>[3x]MKLPVREFDAVVIGAGGAGMRAALQISQSGQTCALLSKVFPTRSHTVSAQGGITVALGNTHEDNWEWHMYDTVKGSDYIGDQDAIEYMCKTGPEAILELEHMGLPFSRLDDGRIYQRPFGGQSKNFGGEQAARTAAAADRTGHALLHTLYQQNLKNHTTIFSEWYALDLVKNQDGAVVGCTALCIETGEVVYFKARATVLATGGAGRIYQSTTNAHINTGDGVGMAIRAGVPVQDMEMWQFHPTGIAGAGVLVTEGCRGEGGYLLNKHGERFMERYAPNAKDLAGRDVVARSIMIEIREGRGCDGPWGPHAKLKLDHLGKEVLESRLPGILELSRTFAHVDPVKEPIPVIPTCHYMMGGIPTKVTGQALTVNEKGEDVVVPGLFAVGEIACVSVHGANRLGGN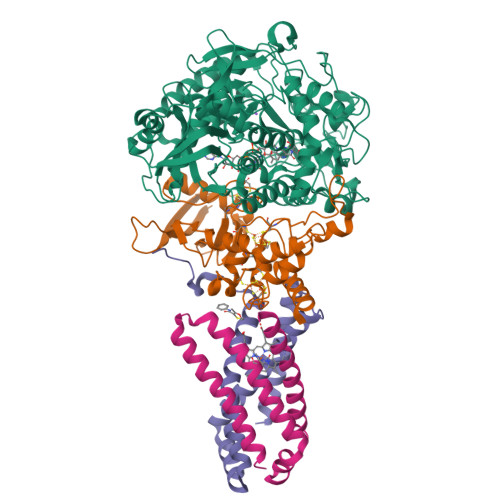SLLDLVVFGRAAGLHLQESIAEQGALRDASESDVEASLDRLNRWNNNRNGEDPVAIRKALQECMQHNFSVFREGDAMAKGLEQLKVIRERLKNARLDDTSSEFNTQRVECLELDNLMETAYATAVSANFRTESRGAHSRFDFPDRDDENWLCHSLYLPESESMTRRSVNMEPKLRPAFPPKIRTY;>[3x]MRLEFSIYRYNPDVDDAPRMQDYTLEADEGRDMMLLDALIQLKEKDPSLSFRRSCREGVCGSDGLNMNGKNGLACITPISALNQPGKKIVIRPLPGLPVIRDLVVDMGQFYAQYEKIKPYLLNNGQNPPAREHLQMPEQREKLDGLYECILCACCSTSCPSFWWNPDKFIGPAGLLAAYRFLIDSRDTETDSRLDGLSDAFSVFRCHSIMNCVSVCPKGLNPTRAIGHIKSMLLQRNA;>[3x]MIRNVKKQRPVNLDLQTIRFPITAIASILHRVSGVITFVAVGILLWLLGTSLSSPEGFEQASAIMGSFFVKFIMWGILTALAYHVVVGIRHMMMDFGYLEETFEAGKRSAKISFVITVVLSLLAGVLVW;>MVSNASALGRNGVHDFILVRATAIVLTLYIIYMVGFFATSGELTYEVWIGFFASAFTKVFTLLALFSILIHAWIGMWQVLTDYVKPLALRLMLQLVIVVALVVYVIYGFVVVWGV[3x]>MWSHPQFEKGSGGSGMSAVSGFTPSGQKRSLAELLDGRVKRLDRKSNNSVLQEAALYLLSCNQDVSQFLSEVEAPPYKKTCNPENPVSIKSRMPSAAFVGSTLKDQASCLKISPGILTAKAAVANIQQICQACGDSSAVLNPEQREKLCSLLKTLKILLAENCFCRSLFCKEIWIHRPPLVFEAVWHLHNEGIVCLDEILESCKDTISAVDWLFSEMCSLCLYIDNSSLAGDLAEKMISDFQALLVENSFRRSSATERILEQHKTEEICLSILDKLLSWLLDAVSVEKSDKSSAEQHWLSAFEVHRYRARVVPESIEQFFIHTLTQVLTFKPKLKVSDAIQCQANWSFVKTSTLLTDLYRKLFVALSAEKLIAHIQLVLDTQEVNWHHVLTCVSCLVICLPEAQQLIKDLLCRLLTHAFESYELEGMITAFLIVRQAALEGPAAFVSYTEWFKCTFGAANSYHGNSKKSLVFLLKFLSDIVPFEAPQYLKVHVLHPPFVPTKYRPLLMEYISLAKTRLTDMKVSIEDMGLYEDLSARSNKVQPESQAHQDVEKALNIFENTGKIPASVMEASIFRRPYFTSRFLPALLTPRVLPAAPDALMLLIDSMKRADKIPTNMFNAYIEACEQEKLRKQKGRQ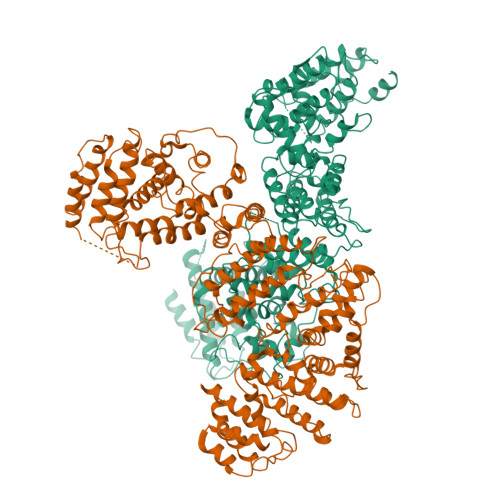QMDQSLPDEPLGILQSALSDLRPLVTDANKYEDVSAQVAVISEKLIAVMGEQKVDDDQVAAKFLKLEDGAQLDIQEQTVADLLLTCFCQCLIAASGTNPPDRQGQWPTLYVKMLCGHQWAFAAVLRRMLQLLRFQAPFLKDSHIVGLAAFSIHLHECQPSLQFLITGVQNLEHYWENLLNLLCSDSVGVCLKLCTAAISYAFCRFSELHQDIFSGCVPPLFLRKLQYLVPRLIWETRGEVIRDDEEADSPLNWNLYALAGWKEAALSLWNQNRLQGLLREKSFQVTFMDWLLWEMTLKSNNDVLCDTDRQEYQRWAVNHYLSESSVVGGCNGDLERGCITIAEAVLQFSNRHIQHSEWESRNISMLKSHTGLGDILCRLQELICDIVTSHHQKGRRHFFFAIFYQRLELHKGKKELSNHLSKQGVLEMCCRILLGLPPLFLINTPSEKGIRTLGSEDFWQFVNKELKNLGPRGYALPYNITAHFFRGVISASVQCKDSSEAVNSILSATYSTCPALLISAAVGWPQLDPVLRSQWCSLFGVDLPKELRTLREQQASVDSCLSQGEKLSLSCTPWLSAAFLYSTVQRKKLPCSRMLEILDGLSSNFSMVLISLLFFSVMDIIYMFLKDGRKHKDLLENCVHIIHCLEQKGETWVWLFQMTDERKPELGLHLHRAASDVFLNLMPFAFFWLVPSLQLEQVVQQQDFLVIALDMYHKFLQLFVDGSPLSSLSAKSHHLDSHDVFTCGRQFLLCCVPKCQKPNSAILKKMLESWEEHDPELAAVLTRSFKAPDDYDDLFFEPVF[2x]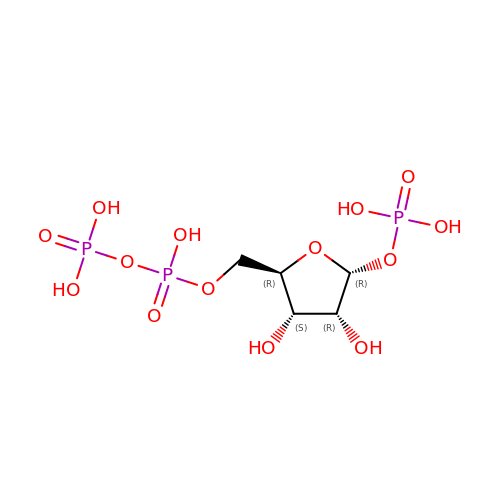5-O-[(R)-hydroxy(phosphonooxy)phosphoryl]-1-O-phosphono-alpha-D-ribofuranose | C5 H13 O14 P3 | FPVTZUUYHCKWRL-TXICZTDVSA-N Shiga toxin (Stx) is the major virulence factor of STEC and is an AB5 toxin consisting of a single A-subunit associated with 5 B-subunits (AB5). The A-subunit encodes an active N-glycosidase that binds to the 60S ribosomal subunit and removes a conserved adenine residue from the 28S rRNA, which inhibits host cell translation and results in cell death. The B-subunit is a receptor-binding protein. Recently, we identified a new subtype of Stx2, designated as Stx2k, in strains isolated from a broad range of hosts in China, including diarrheal patients, goat, pig, and raw meat (beef and mutton).

Considering the difficulty of purifying large quantities of Stx2k from wild type pathogenic bacteria, a recombinant construct encoding a non-toxic toxoid of Stx2k was generated by converting the glutamic acid at position 167 to glutamine (Stx2kE167Q). The E167Q mutation was chosen because E167 is known to be the active site residue for known ribosomal inactivating proteins (RIPs), including the Stxs, and because the E167Q mutation does not alter the structure of RIPs. Molecular-replacement resulted in a solution with two biological units in the crystallographic asymmetric unit. Each biological unit is composed of one A-subunit and five B-subunits. For the A-subunit, residues 243–256 were flexible and could not be located in the electron density map in one of the biological units, and residues 244–257 of the A-subunit in the other biological unit could not be located. As expected, based on sequence identity, the structures of Stx2kE167Q and Stx2a are similar. The most notable similarity was the helix close to the C-terminus of the A-subunit, which was packed in the cavity at the center of the pentameric complex of the B-subunit. Superimposing the active center residues of Stx2a and Stx2kE167Q revealed minimal changes in their spatial configuration, suggesting that any variation in toxin potency may be due to the internalization of the toxins dictated by the B-subunit, rather than the enzymatic activity of the A-subunit. In the crystal structure of Stx2k toxoid, there is a HEPES molecule in the active center of the A-subunit. Residues important for receptor-interaction have been identified by structural studies of Stx2a in complex with its receptor or receptor analogues. These residues constitute three sites for association with the host cell and are conserved between Stx2a and Stx2k except for AA16, which is part of site 1, and AA31, which is part of site 2.

>QEFTIDFSTQQSYVSSLNSIRTAISTPLEHISQGATSVSVINHTPPGSYISVGIRGLDVYQAHFDHLRLIIEQNNLYVAGFVNTATNTFYRFSDFAHISLPGVTTISMTTDSSYTTLQRVAALERSGMQISRHSLVSSYLALMEFSGNTMTREASRAVLRFVTVTAQALRFRQIQREFRQALSETAPVYTMTPEDVDLTLNWGRISNVLPEYRGEDGVRVGRISFNNISAILGTVAVILNCHHQGARSVRAVNEESQPECQITGDRPVIKINNTLWESNTAAAFLNRKSQSLYTTGE[2x];>[10x]ADCAKGKIEFSKYNENDTFTVKVAGKEYWTNRWNLQPLLQSAQLTGMTVTIKSSTCASGSGFAEVQFNND Although the first 3D-structures of Sm assemblies were derived from archaea, the function(s) of Sm-like archaeal proteins (SmAPs) remains unknown. The SmAPs adopt a Sm-fold composed of an N-terminal α-helix and five β-strands. Archaea often possess two SmAP paralogues, SmAP1 and SmAP2, both of which form homo-heptamers, and occasionally rings of different sizes. Several studies revealed that SmAPs from different archaea bind to oligo-U stretches of various lengths.

The crystal structure of Sso-SmAP2 was determined at 2.6 Å resolution. Sso-SmAP2 possesses the classical Sm fold, consisting of an N-terminal helix and five strongly bent strands forming a half-open β-barrel. The heptameric assembly is formed via the outer β-strands, β4 and β5, resulting in a ~12 Å central pore.The overall architecture of the heptameric Sso-SmAP1 and the heptameric Sso-SmAP2 complex is very similar, as the superposition of the two heptameric assemblies yielded a root-mean-square deviation (rmsd) of 1.1 Å for 391 out of 515 superimposed Cα atoms. The major structural differences between both Sso-SmAPs are found in loop L4 and in the N- and C-terminal regions.The extended N-terminus of Sso-SmAP1 forms a protrusion on the L3 face at the proximal site that results in the formation of distinct grooves between the subunits, whereas Sso-SmAP2 displays a smoother surface due to the absence of the N-terminal extension. Interestingly, the corresponding region (Thr40, Asn42, Arg68 and Ser70) of Sso-SmAP2 displays modification(s). Thr40 replaces His40, which is responsible for stacking interactions with the uracil base (magenta). In fact, the methyl group of Thr40 protrudes into the uridine-binding pocket, and thereby most likely interferes with uracil binding. In contrast, the L3 face/proximal site of Sso-SmAP2 is significantly more positively charged due to the presence of Asn7, Lys10 and Arg13. Sso-SmAP2 is predominantly negatively charged, which is effected by residues Asp26, Ser28, Tyr30 and Glu50, whereas the presence of residues Asn29 and Lys30 confers a more positive charge distribution in Sso-SmAP1.

>[7x]GAMDMQAKVENPLKSLRTAINRIVLVKLKDGSEYIGKLEQTDGTMNLVLRDCTEIREGTSEPVAKYGRVLIRGSNILFISVDYETVMNSEK> NLYQFKNMIKCTVPSRSWWDFADYGCYCGRGGSGTPVDDLDRCCQVHDNCYNEAEKISKCWPFFKTYSYKCSQGTLTCKGGNNACAASVCDCDR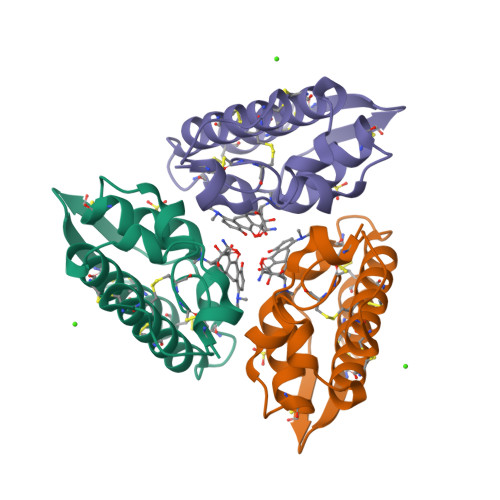LAAICFAGAPYNDNNYNIDLKARCQ>[2x]GAMGNLRLIGVPESDVENGTKLENTLQDIIQENFPNLARQANVQIQEIQR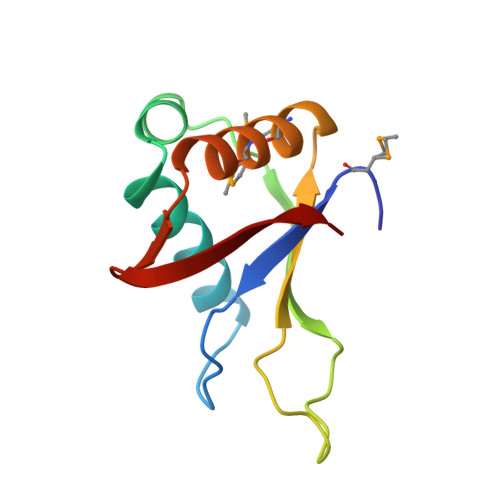TPQRYSSRRATPRHIIVRFTKVEMKEKMLRAAREKGRVTLKGKPIRLTVD>[2x]MAHHGVSGLVGKLVTQLEVNCDADIFYKIVKHHEEVPNVIPHFFTGVQVTKGDGLVSGCIKEWNYVLEGKAMTAVEETTHADETR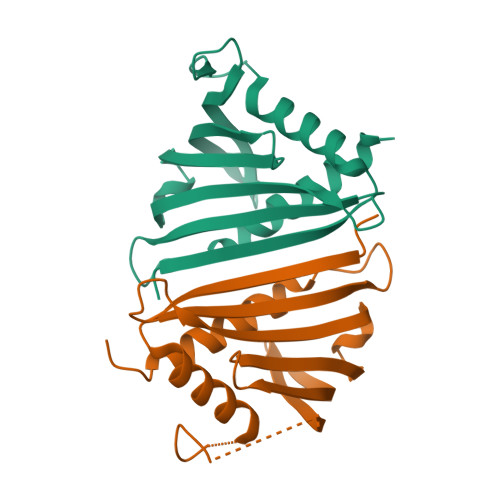TLTHHITEGDAMKDYKKFDVIVETNPKPNGHGSVVTYSIVYEKINEDSPAPFDYLKFFHQNIVDMSAHICSSA> SMRLPERLVEAIAESIIQKLGKEEGILELEDPATFKKKIISLFKEADREEKELEEKAKAVLRENLEVLERENIDYRTAFLAVKRKLAEEMNINVDRRERLNQIINRIMDLIMKDESVEIYEDPPVIRKKIREIVLGALKIEEEIEKTVRQRIKKYSRDLLEGSPEWQILWKRIYEDELKKRGLA

AaDUF507 is a Y-shaped α-helical protein consisting of an anti-parallel 4-helix bundle base and two helical arms that extend 30-Å from the base. The tertiary structure exhibits pseudo-twofold symmetry. Structure-based query of the Protein Data Bank revealed no other protein with a similar tertiary structure, leading us to propose that AaDUF507 represents a new protein fold. In summary, considering the SAXS data, which reports on the oligomeric state at low protein concentration, and the crystal structures, which provide information on oligomeric structure at high protein concentration, we conclude that AaDUF507 is predominantly monomeric in solution.

The two crystal structures differ by a 25° rigid body rotation of the C-terminal arm. The electron density map for the C2221 structure indicated an unknown ligand bound to the protein. The electron density resembled a 6-membered aromatic ring with a small, planar functional group attached. The density could be modeled satisfactorily as nicotinamide, although its true identity is unknown. The unknown ligand site is a pocket located in the junction between the 4-helix bundle and the C-terminal arm, near the intersection of αA, αF, and αG. The ring of the ligand is buried inside the protein and the functional group protrudes out into the solvent. The modeled ligand forms no hydrogen bonds with the protein, as judged by a cutoff distance of 3.2 Å, and appears to be stabilized mainly by nonpolar interactions. With the C-terminal domain rotated as in the C2221 structure, the arms of the Y are closer together and the pocket opens. Docking against the C2221 structure generated six consensus clusters located in the groove between the two helical arms. Cluster 1/4 is unique to the C2221 structure; apparently, the 25° rigid body rotation of the C-terminal arm opens this site.> MGHHHHHHENLYFQMSYSTFPKTKNDALKEPMFFGQPVNVARYDQQKYEVFEKLIEKQLSFFWRPEEIDVSRDRIDYANLPEHEKHIFISNLKYQTLLDSIQGRSPNVALLPLVSIPELETWVETWSFSETIHSRSYTHIIRNIVNDPSVVFDDIVENEYITARAEDIACYYDDLIEYTQYYNLLGEGVHNVGGKPVTVSLRGLKKKLYLCLMCVNVLEAIRFYVSFACSFAFAERELMEGNAKI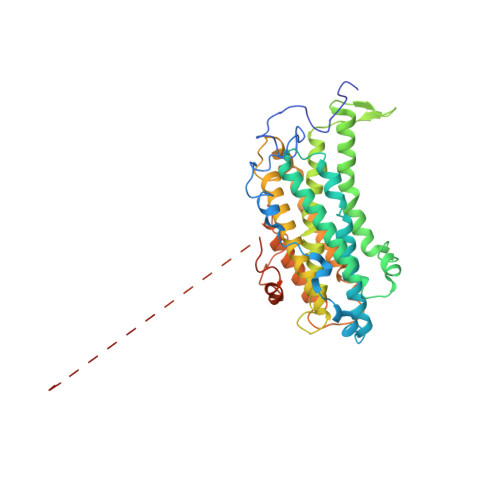IKDIARDEALHLTGTQHMLNLMRSGVDDPEMAEIAAELQDECFQLFKKAAEQEKEWAAYLFKDGSMIGLNKEILSQYVEYITNLRMQAVGLPAGFEGANQNPIPWINAWLSSDNVQVAPQEVEISSYLIGQIDSEVNTDDLGDFEL> MDIEERINLIAQKPTEEILTIDRLKQYLEQGIDLNHYIGFEISGFVHLGTGIISMLKVRDFQKAKVKTTLFLADYHSWINKKLGGDLETIRKVAKGYFAEALKVSLKTVGGDPDEVKVVLGSELYEKLGIEYLENIIKISMNTTLNRIKKGITIMGRKQGESISFAQLLYVPMQVADIYSLNVNLAHGGIDQRKAHVIAIEVSDAFGYKPIAVHHHLLLGMHIDENIRQKLLEAKKTNNRELFEDSVIDIKMSKSKPETAIFIHDTPEDIRRKIRKAYCPIGEIELNPII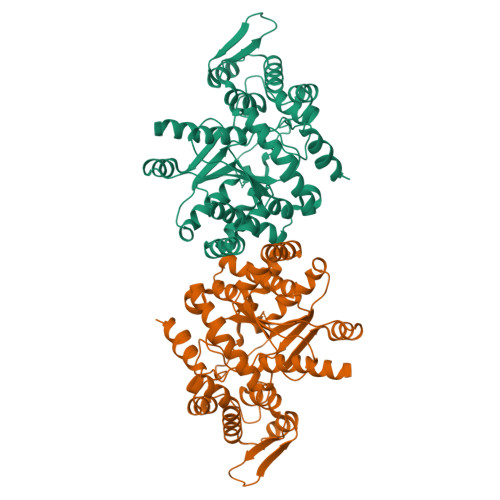ELVEYVIYPILKEPIVIENKKTHQTMEFDNVEQLKEAYAKKQIHPLDLKEYVAEKLIEILEPARKYFLEGKGNKYLEELKNLQITR>MKFKHQGLVADLLPNIRVMQGVGHFMFNYYSEGKKFPHRIYCIVTLLLLLLQYGMMAVNLMMESDDVDDLTANTITMLFFLHPIVKMIYFPVRSKIFYKTLAIWNNPNSHPLFAESNARFHALAITKMRRLLFCVAGATIFSVISWTGITFIEDSVKRITDPETNETTIIPIPRLMIRTFYPFNAMSGAGHVFALIYQFYYLVISMAVSNSLDVLFCSWLLFACEQLQHLKAIMKPLMELSATLDTVVPNSGELFKAGSADHLRESQGVQPSGNGDNVLDVDLRGIYSNRQDFTATFRPTAGTTFNGGVGPNGLTKKQEMLVRSAIKYWVERHKHVVRLVTAVGDAYGVALLLHMLTTTITLTLLAYQATKVNGVNVYAATVIGYLLYTLGQVFLFCIFGNRLIEESSSVMEAAYSCHWYDGSEEAKTFVQIVCQQCQKAMSISGAKFFTVSLDLFASVLGAVVTYFMVLVQLK[3x];> MASILDCPIVSVNARVWRFWSFVLKHDAMRYISIIPVTVMTFFMFTDLCRSWGNIQELIIKAYFAVLYFNAVLRTLILVKDRKLYENFMQGISNVYFEISHIDDHKIQSLLKSYTVRARMLSISNLALGAIISTCFVVYPIFTGERGLPYGMFIPGLDSFRSPHYEIIYIVQVVLTFPGCCMYIPFTSFFASTTLFGLVQIKTLQRQLQTFKDNINSQDKEKVKAKVVKLIEDHKRIITYVSELNSLVTYICFVEFLSFGMMLCALLFLLNVIENHAQIVIVAAYIFMIISQIFAFYWHANEVR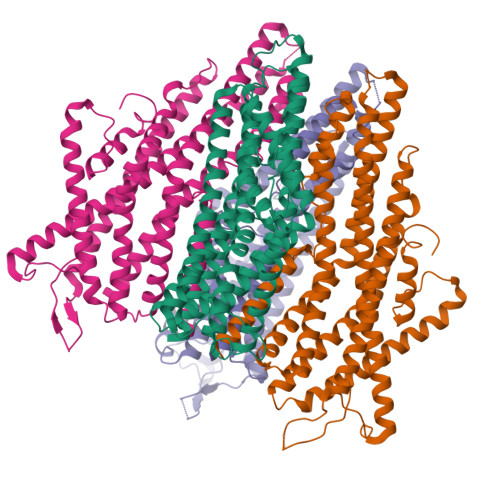EESMNLAEAAYSGPWVELDNSIKKKLLLIILRAQQPLEITVGNVYPMTLEMFQSLLNASYSYFTLLRRVYN>YAPSALVLTVGQGDKAASAGVQRAVTLNCMPKPSGTHPDARGACDQLRAASGNFAEITKIKSGTACTKEWNPFVVTAEGVWEGQRVKYEHTFA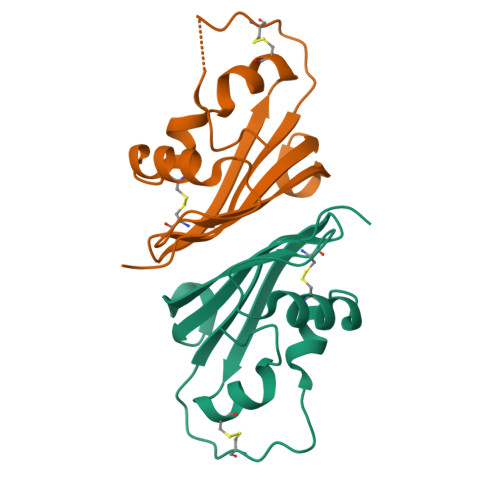NPCEMKAGKGTVFEF[2x]>[10x]APADNAADARPVDVSVSIFINKIYGVNTLEQTYKVDGYIVAQWTGKPRKTPGDKPLIVENTQIERWINNGLWVPALEFINVVGSPDTGNKRLMLFPDGRVIYNARFLGSFSNDMDFRLFPFDRQQFVLELEPFSYNNQQLRFSDIQVYTENIDNEEIDEWWIRGKASTHISDIRYDHLSSVQPNQNEFSRITVRIDAVRNPSYYLWSFILPLGLIIAASWSVFWLESFSERLQTSFTLMLTVVAYAFYTSNILGRLPYTTVIDQMIIAGYGSIFAAILLIIFAHHRQANGVEDDLLIQRCRLAFPLGFLAIGCVLVIRGITL

During activation of a pentameric ligand-gated ion channel (pLGIC), the binding of agonists promotes the opening of a selective ion conduction pore at a distance of more than 50 Å away from the binding sites. Each subunit consists of a predominantly β-stranded extracellular domain and an α-helical transmembrane pore, which interact via an extended interface. Whereas ELIC forms a cation-selective channel with high conductance that is activated with high efficacy by the primary amines cysteamine, propylamine, and GABA, the cation-selective GLIC is activated by protons and inhibited by bulky positively charged compounds that also act as open channel blockers of the nAChR. Our study has identified a cluster of interacting residues located at the β1-β2 turn, the β6-β7 loop and the pre-M1 region of the extracellular domain, and the M2-M3 loop of the pore that exert a strong influence on channel function.

To avoid residual side chain interactions with the ligand-binding domain that may still be present after replacing the proline by alanine, we next investigated the mutation of the respective proline residue in both channels to glycine. In ELIC, the mutation P254G has a small but significant effect on the structure, which overall shows the frequently observed nonconducting conformation. The reorganization of the well-structured M2-M3 loop indicates a change in the conformational properties of this region. In ELIC, the mutant P254G shows agonist-induced currents with a similar EC50 as WT but with a slower activation and an unusually slow deactivation of the channel upon washout of the ligand. This behavior can be observed in two-electrode voltage clamp recordings, where the activity of the protein after a change to ligand-free solution decays slowly, and it becomes even more pronounced in macroscopic recordings of excised outside-out patches. The cause for this unusual deactivation phenotype was revealed in the structure of the P254G mutant of ELIC. In this structure, electron density between Arg255 on the M2-M3 loop and Glu155 located in the β8-β9 loop of the extracellular domain of an adjacent subunit indicates the formation of a strong ionic interaction that is absent in WT and that may stabilize the open conformation of the pore. In the background of the mutation R255A, the kinetics of channel deactivation of the P254G mutant becomes similar to WT, thus confirming the role of the interaction for the unusual functional behavior. Whereas the predominantly local effects of most mutations, which modulate the open to closed equilibrium of the channel, resembles the behavior of eukaryotic receptors, the mutation of a conserved proline (Pro254) to glycine in ELIC resulted in the formation of novel interactions between residues apart from the site of mutation that were not present in WT, causing an unusual functional phenotype that would have been difficult to explain in the absence of structure.>[2x]MVRDMK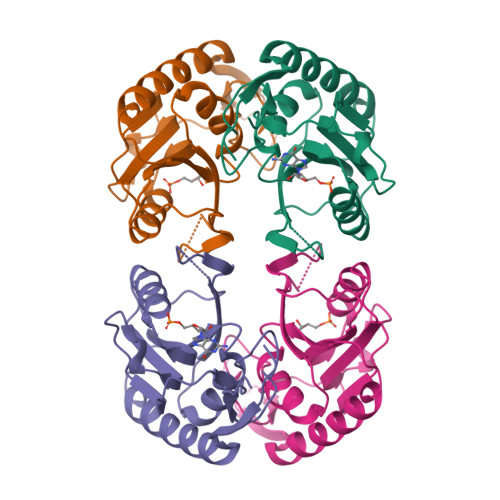HTVEVMIPEAEIKARIAELGRQITERYKDSGSDMVLVGLLRGSFMFMADLCREVQVSHEVDFMTASSYGSGMSTTRDLKILKDLDEDIRGKDVLIVEDIIDSGNTLSKVREILSLREPKSLAICTLLDKPSRREVNVPVEFIGFSIPDEFVVGYGIDYAQRYRHLPYIGKVILLDE>[2x]SNAMAANRMRPI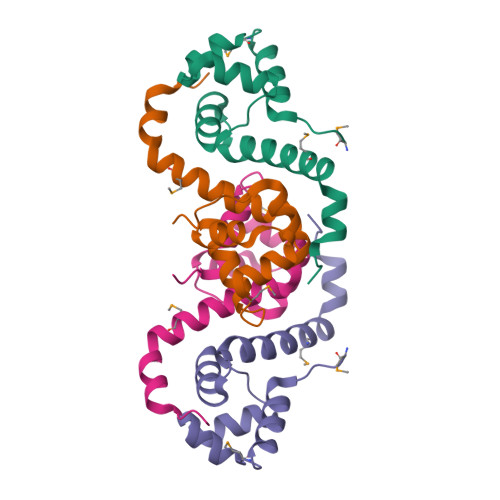HPGEILAEELGFLDKMSANQLAKHLAIPTNRVTAILNGARSITADTALRLAKFFGTTPEFWLNLQDAYDIKMALKKSGKKIEKEVTPYDQAA> GPLGSKK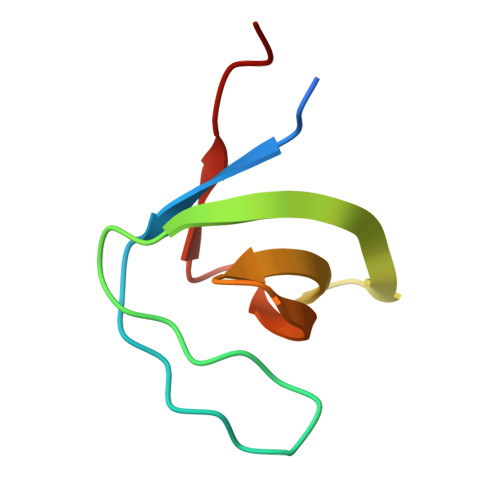RQCKVLFEYIPQNEDELELKVGDIIDINEEVEEGWWSGTLNNKLGLFPSNFVKELEVT>[3x]MEKFVLSLDEGTTSARAIIFDRESNIHGIGQYEFPQHYPRPGWVEHNPEEIWDAQLRAIKDAIQSARIEPNQIAAIGVTNQRETTLVWDKDGKPLYNAIVWQCRRTAEMVEEIKREYGTMIKEKTGLVPDAYFSASKLKWLLDNVPGLREKAEKGEVMFGTVDTFLIYRLTGEHVTDYS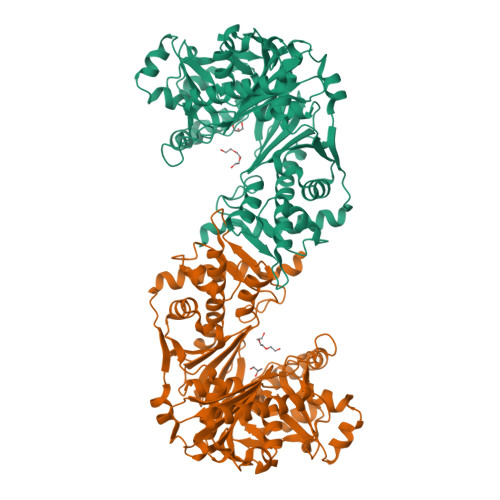NASRTMLFNIKKLDWDDELLELFDIPESVLPEVRESSEVYGYTKKELLGAEIPVSGDAGDQQAALFGQAAFEAGMVKATYGTGSFILVNTDEMVLYSDNLLTTIAWGLNGRVSYALEGSIFVTGAAVQWLRDGIKIIKHASETEELATKLESNEGVYFVPAFVGLGAPYWDQFARGIIIGITRGTGREHLARATLEAIAYLTRDVVDEMEKLVQIKELRVDGGATANDFLMQFQADILNRKVIRPVVKETTALGAAYLAGLAVDYWADTREIAELWKAERIFEPKMDEKTRERLYKGWKEAVKRAMGWAKVVDSAKSN;> MEKFVLSLDEGTTSARAIIFDRESNIHGIGQYEFPQHYPRPGWVEHNPEEIWDAQLRAIKDAIQSARIEPNQIAAIGVTNQRETTLVWDKDGKPLYNAIVWQCRRTAEMVEEIKREYGTMIKEKTGLVPDAYFSASKLKWLLDNLPGLREKAEKGEVMFGTVDTFLIYRLTGEHVTDYSNASRTMLFNIKKLDWDDELLELFDIPESVLPEVRESSEVYGYTKKELLGAEIPVSGDAGDQQAALFGEAAFEAGMVKATYGTGSFILVNTDEMVLYSDNLLTTIAWGLNGRVSYALEGSIFVTGAAVQWLRDGIKIIKHASETEELATKLESNEGVYFVPAFVGLGAPYWDQFARGIIIGITRGTGREHLARATLEAIAYLTRDVVDEMEKLVQIKELRVDGGATANDFLMQFQADILNRKVIRPVVKETTALGAAYLAGLAVDYWADTREIAELWKAERIFEPKMDEKTRERLYKGWKEAVKRAMGWAKVVDSAKSN>MQEEDLPRPSISAEPGTVIPLGSHVTFVCRGPVGVQTFRLERESRSTYNDTEDVSQASPSESEARFRIDSVSEGNAGPYRCIY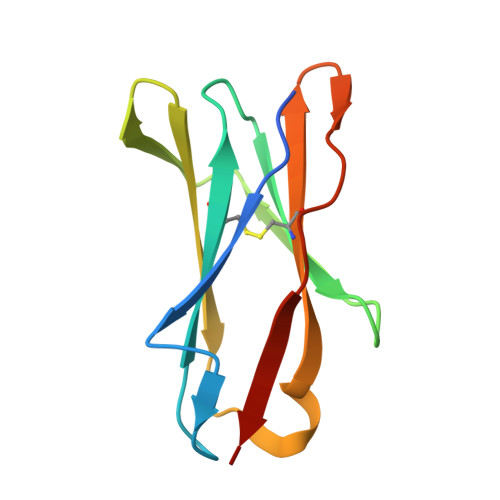YKPPKWSEQSDYLELLVKET[4x]>MGSSHHHHHHSSGLVPRGSHMPATHHSSATSAERPTVVGRIPVLDVRPVVQRGRRPAKAVTGESFEVSATVFREGHDAVGANVVLRDPRGRPGPWTPMRELAPGTDRWGATVTAGETGTWSYTVEAWGDPVTTWRHHARIKIPAGLDTDLVLEEGARLYERAAADVPGREDRRELLAAVDALRDESRPAASRLAAALTPQVDAVLARHPLRDLVTSSDPLPLLVERERALYGAWYEFFPRSEGTPHTPHGTFRTAARRLPAIAAMGFDVVYLPPIHPIGTTHRKGRNNTLSATGDDVGVPWAIGSPEGGHDSIHPALGTLDDFDHFVTEAGKLGLEIALDFALQCSPDHPWVHKHPEWFHHRPDGTIAHAENPPKKYQDIYPIAFDADPDGLATETVRILRHWMDHGVRIFRVDNPHTKPVAFWERVIADINGTDPDVIFLAAAFTRPAMMATLAQIGFQQSYTYFTWRNTKQELTEYLTELSGEAASYMRPNFFANTPDILHAYLQHGGRPAFEVRAVLAATLSPTWGIYSGYELCENTPLREGSEEYLDSEKYQLKPRDWTRAAREGTTIAPLVTRLNTIRRENPALRQLRDLHFHPTDKEEVIAYSKRQGSN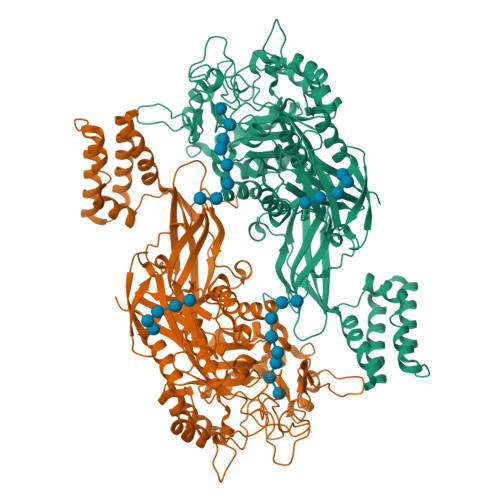TVLVVVNLDPRHTQEATVSLDMPQLGLDWHESVPVRDELTGETYHWGRANYVRLEPGRTPAHVCTVLRPSHPQIGGSHTT[2x]>ACDYTCGSNCYSSSDVSTAQAAGYKLHEDGETVGSNSYPHKYNNYEGFDFSVSSPYYEWPILSSGD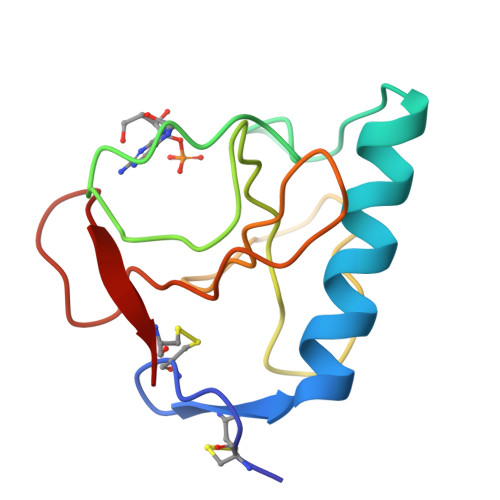VYSGGSPGADRVVFNENNQLAGVITHAGASGNNFVECT[4x]>MYNISFTPDRPLTYHLEDDQSLARLSLVPGRGGLVTEWTVQGQPILYFDRERFQDPSLSVRGGIPILFPICGNLPQDQFNHAGKSYRLKQHGFARDLPWEVIGQQTQDNARLDLRLSHNDATLEAFPFAFELVFSYQLQGHSLRIEQRIANLGDQRMPFSL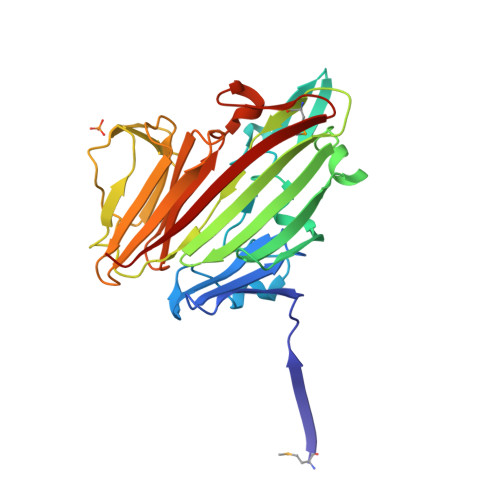GFHPYFFCREKLGITLAIPANDYLDQKTGDCHGYDGQLNLTSPELDLAFTQISQPRAHFIDPDRNLKIEVSFSELYQTLVLWTVAGKDYLCLEPWSGPRNALNSGEQLAWVEPYSSRSAWVNFQVSTE[2x]> GGSKMEYEWKPDEQGLQQILQLLKESQSPDTTIQRTVQQKLEQLNQYPDFNNYLIFVLTKLKSEDEPTRSLSGLILKNNVKAHFQNFPNGVTDFIKSECLNNIGDSSPLIRATVGILITTIASKGELQNWPDLLPKLCSLLDSEDYNTCEGAFGALQKICEDSAEILDSDVLDRPLNIMIPKFLQFFKHSSPKIRSHAVACVNQFIISRTQALMLHIDSFIENLFALAGDEEPEVRKNVCRALVMLLEVRMDRLLPHMHNIVEYMLQRTQDQDENVALEACEFWLTLAEQPICKDVLVRHLPKLIPVLVNGMKYS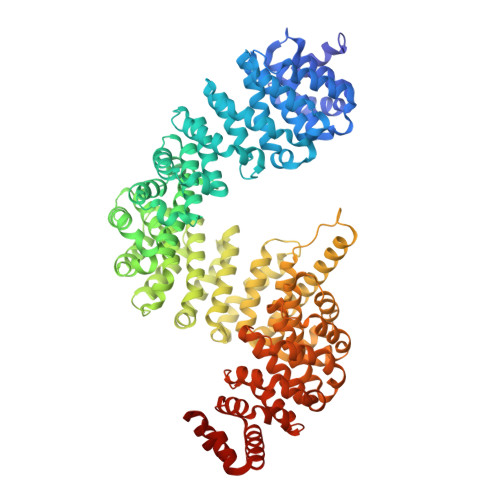DIDIILLKGDVEEDETIPDSEQDIRGGSGGSGDTISDWNLRKCSAAALDVLANVYRDELLPHILPLLKELLFHHEWVVKESGILVLGAIAEGCMQGMIPYLPELIPHLIQCLSDKKALVRSITCWTLSRYAHWVVSQPPDTYLKPLMTELLKRILDSNKRVQEAACSAFATLEEEACTELVPYLAYILDTLVFAFSKYQHKNLLILYDAIGTLADSVGHHLNKPEYIQMLMPPLIQKWNMLKDEDKDLFPLLECLSSVATALQSGFLPYCEPVYQRCVNLVQKTLAQAMLNNAQPDQYEAPDKDFMIVALDLLSGLAEGLGGNIEQLVARSNILTLMYQCMQDKMPEVRQSSFALLGDLTKACFQHVKPCIADFMPILGTNLNPEFISVCNNATWAIGEISIQMGIEMQPYIPMVLHQLVEIINRPNTPKTLLENTAITIGRLGYVCPQEVAPMLQQFIRPWCTSLRNIRDNEEKDSAFRGICTMISVNPSGVIQDFIFFCDAVASWINPKDDLRDMFCKILHGFKNQVGDENWRRFSDQFPLPLKERLAAFYGV>[2x]MAHHHHHHNLNEDYKNKVKGILNKAADDQETTSADTNSNAAKNIPIADNDKVAAELKKQSQAAKTVAAAPNKGSQNQPQTTPNKGSQNQQAAPSPQLQSLSFSADLSNLPKTTAARAASLTKQRIPIQAVTTVPGNTRTFNSRNSGLPTFALNYS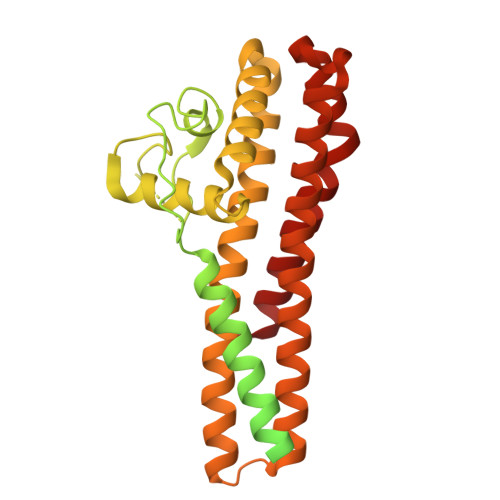FSQPTRQQTNSSSAVQTTTSSGSKLQTLKNELIRAISEEKNKTQNNFGFRETYDQFKMKDSAFELLDVISSAKVYDRSYAPQLNSNTPEAENERNKFYALMDFDQYKIEQFGSIMETLYNENQNHSLIRELMISGLGTQISFELALEEINKKIEIFNQDYLNAKINSFDFTMKLKELKSKLNQILDKRKEWSRQADGLIANASSNSSLSDSKSLAEYIKKRYLDNMQNARQSVLEAYISIM4-{1-[2-chloro-6-(trifluoromethyl)benzoyl]-4-fluoro-1H-indazol-3-yl}-3-fluorobenzoic acid | C22 H10 Cl F5 N2 O3 | 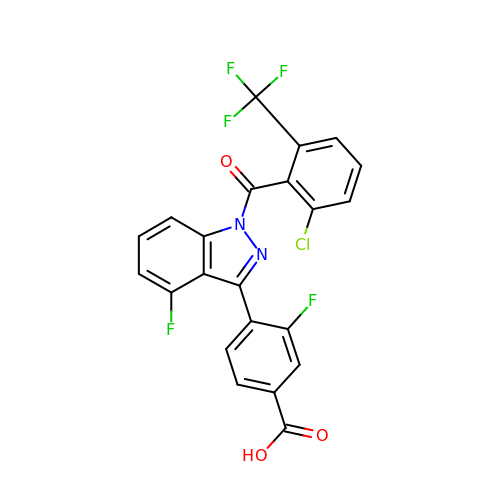PFVOSXMQCIFOSO-UHFFFAOYSA-N>[60x]MGSSHH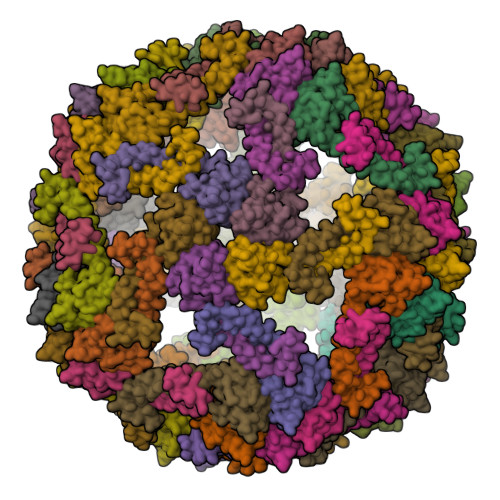HHHHSQDPKNIKIMRLVTGEDIIGNISESQGLITIKKAFVIIPMQATPGKPVQLVLSPWQPYTDDKEIVIDDSEVITITSPKDDIIKSYESHTRVLENKQVEEILRLEKEIEDLQRMKEQQELSLTEASLQKLQERRDQELRRLEEE>GSHMASMKFAVIDRKNFTLIHFEIEKPIKPEILKEIEIPSVDTRKGVVISGRGPIWLHCFLAHKYHHTPFVAVYDPRLGAVVVQSHSELREGDVIDVVVEEILKGGVR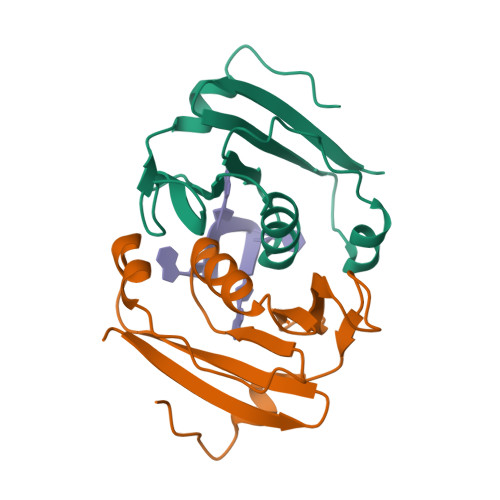HV[2x]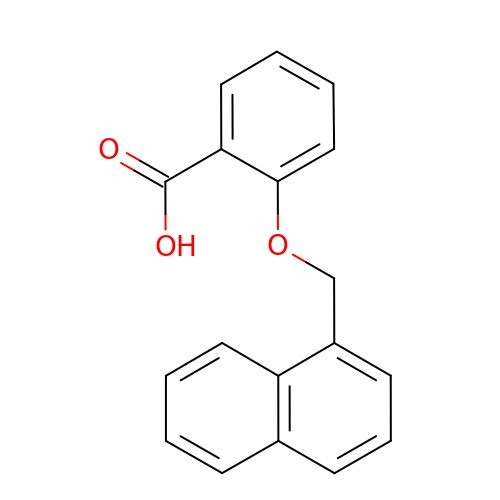2-(naphthalen-1-ylmethoxy)benzoic acid | C18 H14 O3 | MDMYMMOPBHNQFV-UHFFFAOYSA-N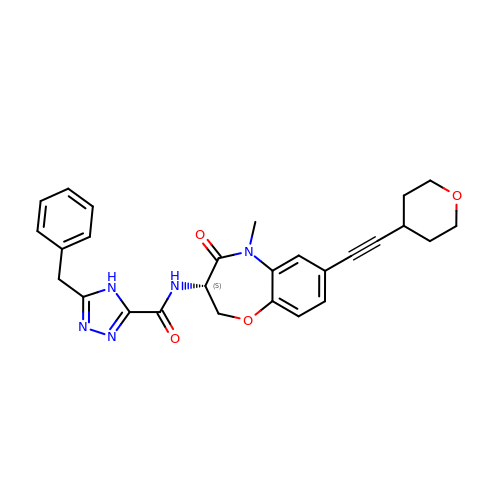N-[(3S)-5-methyl-7-[2-(oxan-4-yl)ethynyl]-4-oxidanylidene-2,3-dihydro-1,5-benzoxazepin-3-yl]-5-(phenylmethyl)-4H-1,2,4-triazole-3-carboxamide | C27 H27 N5 O4 | LIXYKOPHOIRESO-NRFANRHFSA-N> MANRQHVISVDLRLLTGNFDSSLNYIQGRLNGVFGVVSDNATNSFFGNGGFLSSYLWNQAFNAIQMAGIAAFRAIGNEVKRAISYQDNLISMATSYKGLLNLTTKEAFGLARESNIIFQQRNVGLPTFGNFGTQLRAQYGDDFLSAFYDQNNMKGSLERTADMIGRTTVLLGSISGVTNYQRTSFLSNFLSDDFKKLQRLEVFRNSPQLQRAFNSQVDSIGGEQGFNALTRKDRLLLLENIAAIAVDDDIIKAYKDSLGGVLSRLGQELFGDIGIFSFTRDLIFGLPNTSILNSITFFMKEVFAPDGVFGLIKPALQGIVDTVLIGTKFILDRTSFIFMGLN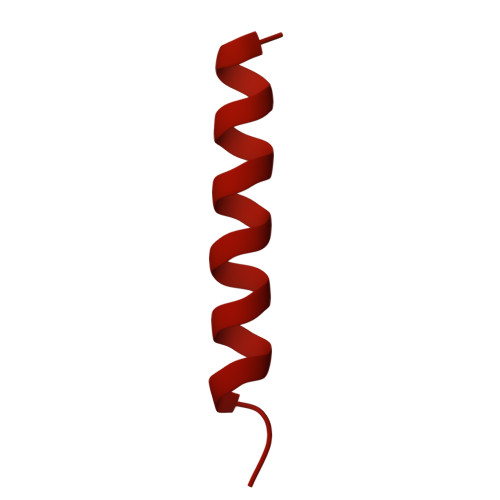ALARVLQPIAPLIYATSSALTVLAAVGLANTIKSAVQGYLISSGAAMLGGRMGMAAMFGMGGDLVGLKTLGTLGLGKLIAPLGFLTMGLDKLADVGWLAISGGFAKAALGIKTFGMSLWAIVANPAFLTIAGIVGAIALAGYTLWKYWEPIGDFLQGFWIGFKAGLPILDQIESVLQSIGQALSPITEGFKNMASAMQPVLDGFTKFFNLQQEKGGENYVKQGVNFGDAASGVTRTILSNPLINPFSGFFGLFGNPAQNKADGDPQSVMSAINDERRKMPSGASLVIANSSENVFTRSQTQQLASAGRGSTVINNTFNISGADPQAIAKQIADIINSQWQGTLTDYA> MVARVQTAEEIRDEGNAAVKDQDYIKADELYTEALQLTTDEDKALRPVLYRNRAMARLKRDDFEGAQSDCTKALEFDGADVKALFRRSLAREQLGNVGPAFQDAKEALRLSPNDKGIVEVLQRLVKANNDKIKQTTSLANKVTDMEKLAFRGEAKDTEQKMTALNNLLVLCRESESGATGVWNQGALVPFVLNLINDASENEEVTVTAIRILDETIKNSVRCMKFLAMHDPDGPKSVRFVCRLMCKKSTKDFVDATGILVQRVFNAMAKMDRQKEMKPDPEVAEANKIWIIRVLLELQEMLQDPKVGAVQRETCIDLFLKNLMHMDGGIPRGWSWKFVEERGLLALLDVASQIPELCEYPVSAETRQHVAICLQRLEEDMVFDTKRTIFKEKVDMFFNALISRCTNDDEGHKYRIKLSCFLITMLQGPVDIGINLITNDQLTPIMLEMAASQDHLMQGIAAELIVATVSKHERAINMLKVGIPVLRALYDSEDPTVKVRALVGLCKIGAAGGDDISKATMKEEAVISLAKTCKKFLLETEKYSVDIRRYACEGLSYLSLDADVKEWIVDDSLLLKALVLLAKKAGALCVYTLATIYANLSNAFEKPKVDEEMVKLAQFAKHHVPETHPKDTEEYVEKRVRALVEEGAVPACVAVSKTESKNALELIARSLLAFAEYEDLRGRIIAEGGTVLCLRLTKEASGEGKIKAGHAIAKLGAKADPMISFPGQRAYEVVKPLCDLLHPDVEG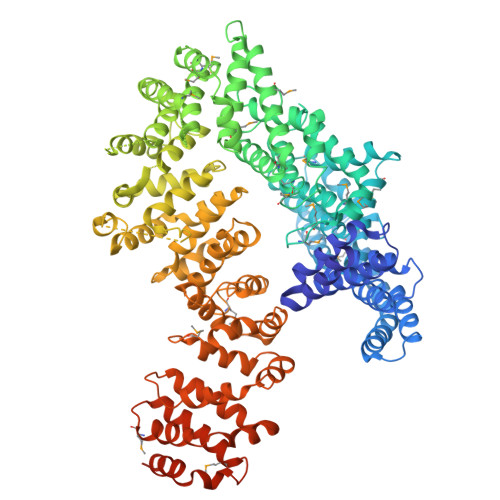KANYDSLLTLTNLASVSDSIRGRILKEKAIPKIEEFWFMTDHEHLRAAAAELLLNLLFFEKFYEETVAPGTDRLKLWVLYSAEVEEERLSRASAAGFAILTEDENACARIMDEIKSWPEVFKDIAMHEDAETQRRGLMGIANIMHSSNKLCSEIVSSEVFRVLVAVTKLGTINQERAGSTEQAKRGLEAAEKFGLIKATDREIYERENQMSTIQE>MAEESRGQRGSGYGLGLSTRTQVTGYQFLARRTAMALTRWRVRMEIEPGRRQTLAVVASVSAALVICLGALLWSFISPSGQLNESPIIADRDSGALYVRVGDRLYPALNLASARLITGRPDNPHLVRSSQIATMPRGPLVGIPGAPSSFSPKSPPASSWLVCDTVATSSSIGSLQGVTVTVIDGTPDLTGHRQILSGSDAVVLRYGGDAWVIREGRRSRIEPTNRAVLLPLGLTPEQVSQARPMSRALFDALPVGPELLVPEVPNAGGPATFPGAPGPIGTVIVTPQISGPQQYSLVLGDGVQTLPPLVAQILQNAGSAGNTKPLTVEPSTLAKMPVVNRLDLSAYPDNPLEVVDIREHPSTCWWWERTAGENRARVRVVSGPTIPVAATEMNKVVSLVKADTSGRQADQVYFGPDHANFVAVTGNNPGAQTSESLWWVTDAGARFGVEDSKEARDALGLTLTPSLAPWVALRLLPQGPTLSRADALVEHDTLPMDMTPAELVVPK[6x];>[6x]MKRGFARPTPEKPPVIKPENIVLSTPLSIPPPEGKPWWLIVVGVVVVGLLGGMVAMVFASGSHVFGGIGSIFPLFMMVGIMMMMFRGMGGGQQQMSRPKLDAMRAQFMLMLDMLRETAQESADSMDANYRWFHPAPNTLAAAVGSPRMWERKPDGKDLNFGVVRVGVGMTRPEVTWGEPQNMPTDIELEPVTGKALQEFGRYQSVVYNLPKMVSLLVEPWYALVGEREQVLGLMRAIICQLAFSHGPDHVQMIVVSSDLDQWDWVKWLPHFGDSRRHDAAGNARMVYTSVREFAAEQAELFAGRGSFTPRHASSSAQTPTPHTVIIADVDDPQWEYVISAEGVDGVTFFDLTGSSMWTDIPERKLQFDKTGVIEALPRDRDTWMVIDDKAWFFALTDQVSIAEAEEFAQKLAQWRLAEAYEEIGQRVAHIGARDILSYYGIDDPGNIDFDSLWASRTDTMGRSRLRAPFGNRSDNGELLFLDMKSLDEGGDGPHGVMSGTTGSGKSTLVRTVIESLMLSHPPEELQFVLADLKGGSAVKPFAGVPHVSRIITDLEEDQALMERFLDALWGEIARRKAICDSAGVDDAKEYNSVRARMRARGQDMAPLPMLVVVIDEFYEWFRIMPTAVDVLDSIGRQGRAYWIHLMMASQTIESRAEKLMENMGYRLVLKARTAGAAQAAGVPNAVNLPAQAGLGYFRKSLEDIIRFQAEFLWRDYFQPGVSIDGEEAPALVHSIDYIRPQLFTNSFTPLEVSVGGPDIEPVVAQPNGEVLESDDIEGGEDEDEEGVRTPKVGTVIIDQLRKIKFEPYRLWQPPLTQPVAIDDLVNRFLGRPWHKEYGSACNLVFPIGIIDRPYKHDQPPWTVDTSGPGANVLILGAGGSGKTTALQTLICSAALTHTPQQVQFYCLAYSSTALTTVSRIPHVGEVAGPTDPYGVRRTVAELLALVRERKRSFLECGIASMEMFRRRKFGGEAGPVPDDGFGDVYLVIDNYRALAEENEVLIEQVNVIINQGPSFGVHVVVTADRESELRPPVRSGFGSRIELRLAAVEDAKLVRSRFAKDVPVKPGRGMVAVNYVRLDSDPQAGLHTLVARPALGSTPDNVFECDSVVAAVSRLTSAQAPPVRRLPARFGVEQVRELASRDTRQGVGAGGIAWAISELDLAPVYLNFAENSHLMVTGRRECGRTTTLATIMSEIGRLYAPGASSAPPPAPGRPSAQVWLVDPRRQLLTALGSDYVERFAYNLDGVVAMMGELAAALAGREPPPGLSAEELLSRSWWSGPEIFLIVDDIQQ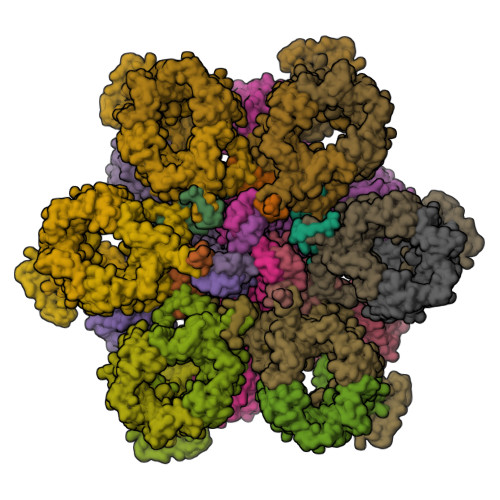LPPGFDSPLHKAVPFVNRAADVGLHVIVTRTFGGWSSAGSDPMLRALHQANAPLLVMDADPDEGFIRGKMKGGPLPRGRGLLMAEDTGVFVQVAATEVRR;>MTAVADAPQADIEGVASPQAVVVGVMAGEGVQIGVLLDANAPVSVMTDPLLKVVNSRLRELGEAPLEATGRGRWALCLVDGAPLRATQSLTEQDVYDGDRLWIRFIADTERRSQVIEHISTAVASDLSKRFARIDPIVAVQVGASMVATGVVLATGVLGWWRWHHNTWLTTIYTAVIGVLVLAVAMLLLMRAKTDADRRVADIMLMSAIMPVTVAAAAAPPGPVGSPQAVLGFGVLTVAAALALRFTGRRLGIYTTIVIIGALTMLAALARMVAATSAVTLLSSLLLICVVAYHAAPALSRRLAGIRLPVFPSATSRWVFEARPDLPTTVVVSGGSAPVLEGPSSVRDVLLQAERARSFLSGLLTGLGVMVVVCMTSLCDPHTGQRWLPLILAGFTSGFLLLRGRSYVDRWQSITLAGTAVIIAAAVCVRYALELSSPLAVSIVAAILVLLPAAGMAAAAHVPHTIYSPLFRKFVEWIEYLCLMPIFPLALWLMNVYAAIRYR[12x]> GSFIDIEFPEWFHEGLSRHQAENLLMGKDIGFFIIRA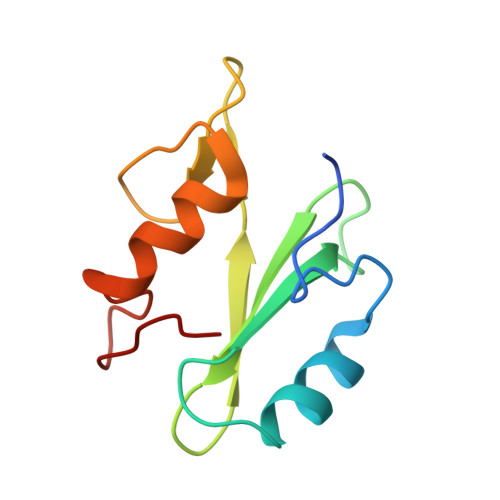SQSSPGDFSISVRHEDDVQHFKVMRDTKGNYFLWTEKFPSLNKLVDYYRTTSISKQKQVFLRD> RPSSRVYIVEVLNEFPHDPYAFTQGLVYAENDTLFESTGLYGRSSVRQVALQTGKVENIHKMDDSYFGEGLTLLNEKLYQVVWLKNIGFIYDRRTLSNIKNFTHQMKDGWGLATDGKILYGSDGTSILYEIDPHTFKLIKKHNVKYNGHRVIRLNELEYINGEVWANIWQTDCIARISAKDGTLLGWILLPNLRKKLIDEGFRDIDV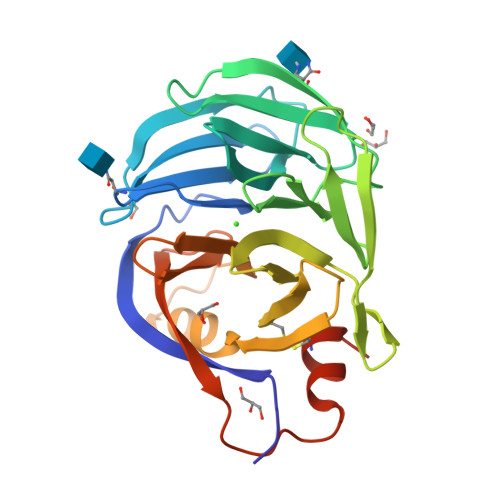LNGIAWDQENKRIFVTGKLWPKLFEIKLHLVRHRIPDGYIERHCLNLRDNTLSLKTDID The anti-proliferative protein Tob belongs to the Tob/BTG family and plays important roles in cell proliferation, embryonic development, cellular differentiation, cancer suppression, and apoptosis. The anti-proliferative mechanism of Tob was revealed by its complex structure complex with CNOT7 (Caf1), and was further shown to be dependent on CNOT7 or CNOT8 but independent of other CCR4-NOT complex subunits. Two conserved regions of Tob, termed Box A and Box B, mediate the largely hydrophobic interaction with CNOT7 and are conserved in other family members, including BTG2. TobN138 consists of five α-helices and four β-strands that form two anti-parallel β-sheets.

We employed a fragment screening approach to discover inhibitors of the Tob-CNOT7 interaction. To provide structural insight into fragment binding, crystals of human Tob residues 1–138 (termed TobN138 hereafter), containing Box A and B motifs, were soaked with a buffer containing several fragments. Structures of TobN138 with two inhibitors, corresponding to compounds 1 (i1) and 6 (i6), were determined to 2.3 Å resolution. In the TobN138-i1 complex, i1 π-stacks against Trp93 and is coordinated by the side-chain of Ser53. Superimposing the Tob-i1 complex onto the Tob-CNOT7 complex structure shows that i1 overlaps with Ser201 and Cys202 on helix α10 of CNOT7. Trp93 is highly conserved among the Tob/BTG family and is located in the Box B motif. Asp95 and Glu98 of Tob form a salt bridge with Lys203 in CNOT7, while Trp93 inserts into a hydrophobic pocket on the CNOT7 surface. The first shows 96.4% inhibition and binds to a strictly conserved site located on Box B in the CNOT7 interface, including residues Trp93 and Asp95. Missense mutations W93A and D95A abolish the interaction between Tob and CNOT7 in vitro and in vivo. Our results indicate that Box B of Tob should be targeted for efficient inhibition of the Tob-CNOT7 interaction.

> HHMQLEIQVALNFIISYLYNKLPRRRVNIFGEELERLLKKKYEGHWYPEKPYKGSGFRCIHIGEKVDPVIEQASKESGLDIDDVRGNLPQDLSVWIDPFEVSYQIGEKGPVKVLYVDDNNENGCELDKEIKNSFNPEAQVFMPISDPASSVSSSPSPPFGHSAAVSPTFMPRSTQPLTFTTATFAATKFGSTKMKNSGRSNKVARTSPINLGLNVNDLLKQKAISSSMHSLYGLGLGSQQQPQQQQQPAQPPPPPPPPQQQQQQKTSALSPNAKEFIFPNMQGQGSSTNGMFPGDSPLNLSPLQYSNAFDVFAAYGGLNEKSFVDGLNFSLNNMQYSNQQFQPVMAN> MLKNEETEKKLNLNQQRLGTVVAVLKSVNAKKVIDLGCGEGNLLSLLLKDKSFEQITGVDVS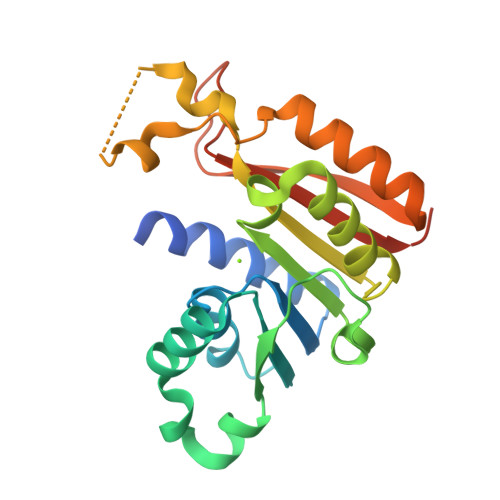YSVLERAKDRLKIDRLPEMQRKRISLFQSSLVYRDKRFSGYDAATVIEVIEHLDENRLQAFEKVLFEFTRPQTVIVSTPNKEYNFHYGNLFEGNLRHRDHRFEWTRKEFQTWAVKVAEKYGYSVRFLQIGEIDDEFGSPTQMGVFTLGAGGHHHHHH>KLPTNLAYERSIDPSDVCFFVVWPDDRKTPLTYNSRTLLGQMEAKSLAYDVSGQPIKSATAEALAQGNPHQVDFCHVPYGASHIECSFSVSFSSELRQPYKCNSSKVKQTLVQLVELYETKIGWTELATRYLMNICNGKWLWKNTRKAYCWNIVLTPWPWNGEKVGFEDIRTNYTSRQDFKNNKNWSAIVEMIKTAFSSTDGLAIFEVRATLHLPTNAMVRPSQVFTEKEAAAAAAAATQNSRVFQSTTIDGERSPILGAFKTGAAIATIDDWYPEATEPLRVGRFGVHREDVTCYRHPSTGKDFFSILQQAEHYIEVLSANKTPAQETINDMHFLMANLIKGGMFQHKGD[6x];> LKEIIASNPDDLTTELKRAFRPLTPHIAIDGNEIDALTILVNLTDKAKCKQKLRDEKWWASCINCVNYRQSHNPKFPDIRSEGVIRTQALGELPSFLLSSSKIPPYHWSYSHDSKYVNKSAFLTNEFCWDGEISCLGELLKDADHPLWNTLKKLGCSQKTCKAMAKQLADITLTTINVTLAPNYLTQISLPDSDTSYISLSPVASLSMQSHFHQRLQDENRHSAITRFSRTTNMGVTAMTCGGAFRMLKSGAKFSSPPHHRLNNGSFLVLPNIRVCGATALSSPVTVGIPSLTAFFGFVHAFERNINRTTSSFRVESFAICVHQLHVEKRGLTAEFVEKGDGTISAPATRDDWQCDVVFSLILNTNFAQHIDQDTLVTSLPKRLARGSAKIAIDDFKHINSFSTLETAIESLPIEAGRWLSLYAQSNNNLSDLLAAMTEDHQLMASCVGYHLLEEPKDKPNSLRGYKHAIAECIIGLINSITFSSETDPNTIFWSLKNYQNYLVVQPRSIN;> KWYYKTITFLPELCNNESLAAKCLRVLHGFNYQYETRNIGVSFPLWCDATVGKKISFVSKNKIELDLLLKQHYFVQMEQLQYFHISNTVLVPEDCTYVSFRRCQSIDKLTAAGLARKIRRLEKRALSRGEAFDPSSFAQKEHTAIAHYHSLGESSKQTNRNFRLNIRMLSEQPREGNSIFSSYGLANSENSFQPVPL;> AMFLQRPKPYSDESLESFFIRVANKNGYGDVHRFLEATKRFLQDIDHNGYQTFPTDITRINPYSAKNSSSARTASFLKLAQLTFNEPPELLGLAINRTNMKYSPSTSAVVRGAEVFPRSLLRTHSIPCCPLCLRENGYASYLWHFQGYEYCHSHNVPLITTCSGHEAACTVSNWLAGHESKPLPNLPKSYRWGLVHWWMGIKDSDHFSFVQFFSNWPRSFHSIIEDEVEFNLEHAVVSTSELRLKDLLGRLFFGSIRLPERNLQHNIILGELLCYLENRLWQDKGLIANLKMNALEATVMLNCSLDQIASMVEQRILKPNRKSKDVTDYLFHFGDIFCLWLAEFQSDEFNRSFYVSRW;> AMFLQRPKPYSDESLESFFIRVANKNGYGDVHRFLEATKRFLQDIDHNGYQTFPTDITRINPYSAKNSSSARTASFLKLAQLTFNEPPELLGLAINRTNMKYSPSTSAVVRGAEVFPRSLLRTHSIPCCPLCLRENGYASYLWHFQGYEYCHSHNVPLITTCSCGKEFDYRVSEAACTVSNWLAGHESKPLPNLPKSYRWGLVHWWMGIKDDHFSFVQFFSNWPRSFHSIIEDEVEFNLEHAVVSTSELRLKDLLGRLFFGSI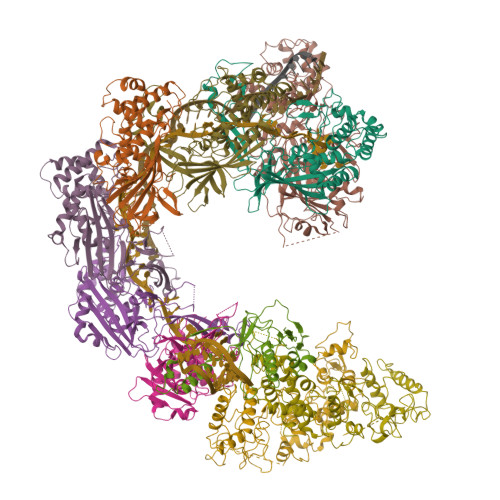RLPERNLQHNIILGELLCYLENRLWQDKGLIANLKMNALEATVMLNCSLDQIASMVEQRILKPNAAAAAAAAADVTDYLFHFGDIFCLWLAAFQSDEFNRSFYVSR1-{(3R)-3-[(7H-pyrrolo[2,3-d]pyrimidin-4-yl)amino]piperidin-1-yl}propan-1-one 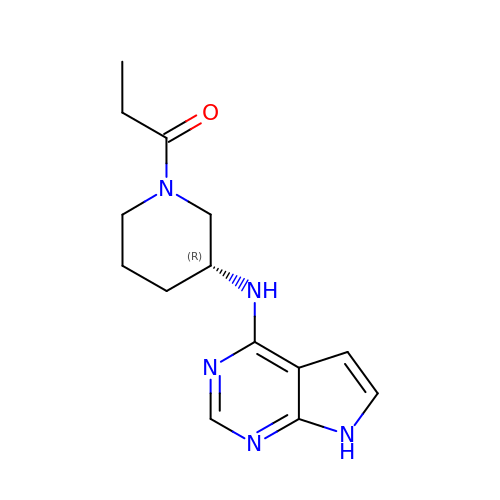| C14 H19 N5 O | HTWQEUNJZRNASZ-SNVBAGLBSA-N>MAITLNSGFKMPVLGLGVWRMDRNEIKNLLLSAINLGYRHFDCAADYKNELEVGEAFKEAFDTDLVKREDLFITTKLWNSDHGHVIEACKNSLKKLQLEYLDLYLIHFPMASKHSGIGTTRSILDDEGVLEVDTTISLEA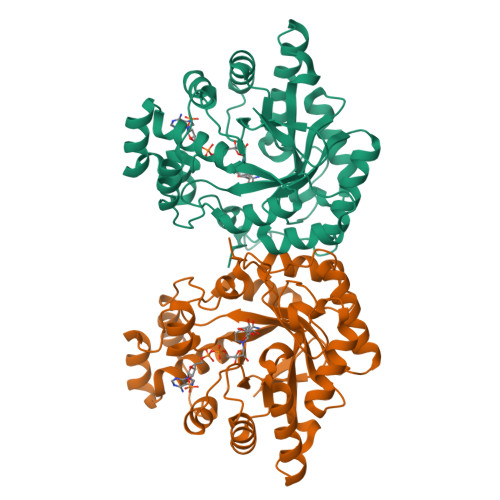TWHEMEKLVEMGLVRSIGISNYDVYLTRDILSYSKIKPAVNQIETHPYFQRDSLIKFCHKYGIAITAHTPLGGALANTERFGSVSCLDDPVLKKLSDKHNKSPAQIVLRWGVQRNTIVIPKSSKTKRLEENLNIFDFELSKEDMELIKTMERNQRSNTPAKAWGIDVYA[4x]>[2x]MNVESKWLEDFLVLAKVKNFSQAAELRNVTQPAFSRRIRLLEDTVGAELVDRKSKPIELTPSGKLFRITARTLVNQIEAGISQISDLSQLGGNVVQVAAAHSLATSLIPKMQQAFDEG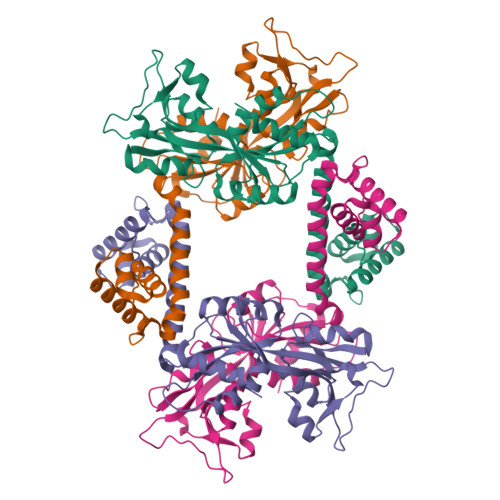DYKPILSVEAIDVDEATKELREGACDILLAFDDDILRLPPYQSQLIAKTELLPVSACDEMGKPIYDFISQGAVPWLTYSSTSYIGRQVEIIREQVALTPIFSSSMTDMLKILVLNKQGIAWLPAYSIQEELAQKKVAIIGEQSLRLPIEYYAYRYQARLHPAGEKVWSILCNLDT>[2x]MQDGWSLAKDAEGIKVYVRNVEGSPLREFRGEVRLK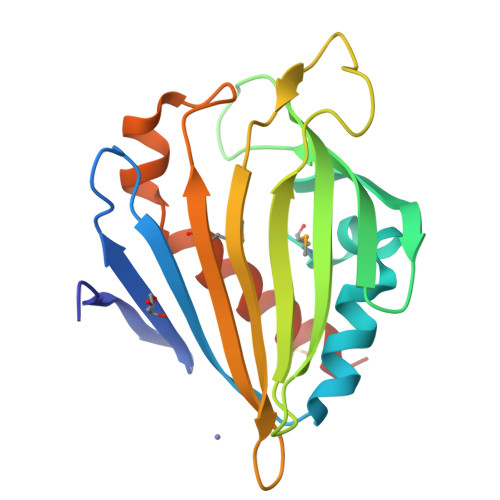AAADDVVKVLRDANAFRQWMPDVAASELLKATDTEQYHYLDNSAPWPVSNRDGVYHFTYEKAGDGAITVRVEAVPDYLPLRKGKVRIPRAKGQWTLVPDADGVDVTYQMHASPGGSIPSWLANQTVVETPFGTLKALRSHLRQAHLEHHHHHH> QISVRGLAGVENVTEL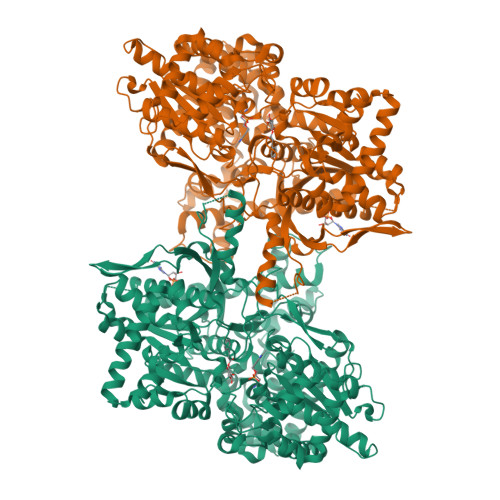KKNFNRHLHFTLVKDRNVATPRDYYFALAHTVRDHLVGRWIRTQQHYYEKDPKRIYYLSLEFYMGRTLQNTMVNLALENACDEATYQLGLDMEELEEIEEDAGLGNGGLGRLAACFLDSMATLGLAAYGYGIRYEFGIFNQKICGGWQMEEADDWLRYGNPWEKARPEFTLPVHFYGRVEHTSQGAKWVDTQVVLAMPYDTPVPGYRNNVVNTMRLWSAKAPNDFNLKDFNVGGYIQAVLDRNLAENISRVLYPNDNFFEGKELRLKQEYFVVAATLQDIIRRFKSSKFGCRDPVRTNFDAFPDKVAIQLNDTHPSLAIPELMRVLVDLERLDWDKAWEVTVKTCAYTNHTVLPEALERWPVHLLETLLPRHLQIIYEINQRFLNRVAAAFPGDVDRLRRMSLVEEGAVKRINMAHLCIAGSHAVNGVARIHSEILKKTIFKDFYELEPHKFQNKTNGITPRRWLVLCNPGLAEIIAERIGEEYISDLDQLRKLLSYVDDEAFIRDVAKVKQENKLKFAAYLEREYKVHINPNSLFDVQVKRIHEYKRQLLNCLHVITLYNRIKKEPNKFVVPRTVMIGGKAAPGYHMAKMIIKLITAIGDVVNHDPVVGDRLRVIFLENYRVSLAEKVIPAADLSEQISTAGTEASGTGNMKFMLNGALTIGTMDGANVEMAEEAGEENFFIFGMRVEDVDRLDQRGYNAQEYYDRIPELRQIIEQLSSGFFSPKQPDLFKDIVNMLMHHDRFKVFADYEEYVKCQERVSALYKNPREWTRMVIRNIATSGKFSSDRTIAQYAREIWGVEPSRQRLPA> AQSVTADPSPPITDTNKLNKYSSRITEPKSQGGSQAILHGVGLSDDDLLKPQIGISSVWYEGNTCNMHLLKLSEAVKEGVENAGMVGFRFNTIGVSDAISMGTRGMCFSLQSRDLIADSIETVMSAQWYDGNISIPGCDKNMPGTIMAMGRLNRPGIMVYGGTIKPGHFQDKTYDIVSAFQSYGEFVSGSISDEQRKTVLHHSCPGAGACGGMYTANTMASAIEAMGMSLPYSSSIPAEDPLKLDECRLAGKYLLELLKMDLKPRDIITPKSLRNAMVSVMALGGSTNAVLHLIAIARSVGLELTLDDFQKVSDAVPFLADLKPSGKYVMEDIHKIGGTPAVLRYLLELGLMDGDCMTVTGQTLAQNLENVPSLTEGQEIIRPLSNPIKETGHIQILRGDLAPDGSVAKITGKEGLYFSGPALVFEGEESMLAAISADPMSFKGTVVVIRGEGPKGGPGMPEMLTPTSAIMGAGLGKECALLTDGRFSGGSHGFVVGHICPEAQEGGPIGLIKNGDIITIDIGAARIDTQVSPEEMNDRRKKWTAPAYKVNRGVLYKYIKNVQSA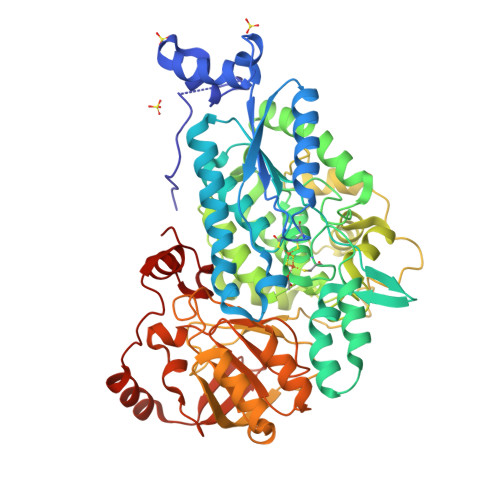SDGCVTDE> GSEGHRTLASTPALWASIPCPRSELRLDLVLPSGQSFRWREQSPAHWSGVLADQVWTLT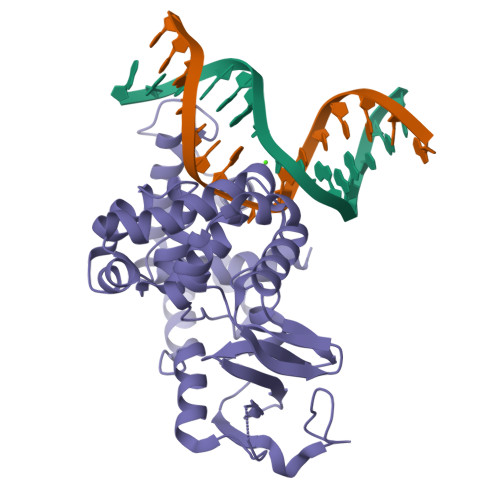QTEEQLHCTVYRGDKSQASRPTPDELEAVRKYFQLDVTLAQLYHHWGSVDSHFQEVAQKFQGVRLLRQDPIECLFSFICSSNNNIARITGMVERLCQAFGPRLIQLDDVTYHGFPSLQALAGPEVEAHLRKLGLGYRARYVSASARAILEEQGGLAWLQQLRESSYEEAHKALCILPGVGTKVADCICLMALDKPQAVPVDVHMWHIAQRDYSWHPTTSQAKGPSPQTNKELGNFFRSLWGPYAGWAQAVLFSADLRQ> SGVDDDMACHKIPVEADFLYAYSTAPGYYSWRNSKDGSWFIQSLCAMLKQYADKLEFMHILTRVNRKVATEFESFS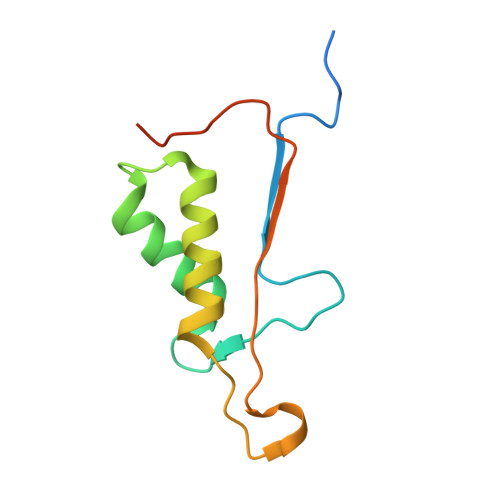FDATFHAKKQIPCIVSMLTKELYFYHLEHHHHHH>[2x]GIEIVLAVSSSVDRKDVVDIINYINEKGIDVWLWLDADKVEEAIELIEEAVKAGVKGIVLRTKKLKLEDIK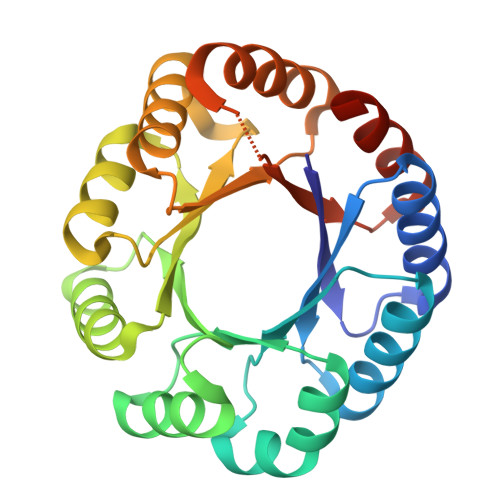KIIDILNKYGVHLLIDTELEEEEIRAIVDLAGPERTTIGLKYDLGEKRERLIRTAVELGVRVLLTDVTDRAQAARGLALAGDRLELLLDVDRTALADLRATLALAAKNPKVGLYLRVSRVDLAARVRAVAAEVADPKRLAFVLDAKNAAEAKALIDALLEHHHHHH> KNTVSIFALGPTITDDDEKMTLALLFLSHSLDNEKQHAQRAGFLVSLLSMAYANPELYLTTNGSNADVKYVIYMIEKDLKRQKYGGFVVKTREMIYEKTTEWIFGSDLDYDQETMLQNGRNNSTIEDLVHTFGYPSCLGALIIQIWIVLVKAITSISGLRKGFFTRLEAFRQDGTVQAGLVLSGDTVDQIGSIMRSQQSLVTLMVETLITMNTSRNDLTTIEKNIQIVGNYIRDAGLASFFNTIRYGIETRMAALTLSTLRPDINRLKALMELYLSKGPRAPFICILRDPIHGEFAPGNYPAIWSYAMGVAVVQNRAMQQYVTGRSYLDIDMFQLGQAVARDAEAQ;> MESDAKNYQIMDSWEEEPRDKSTNISSALNIIEFILSTD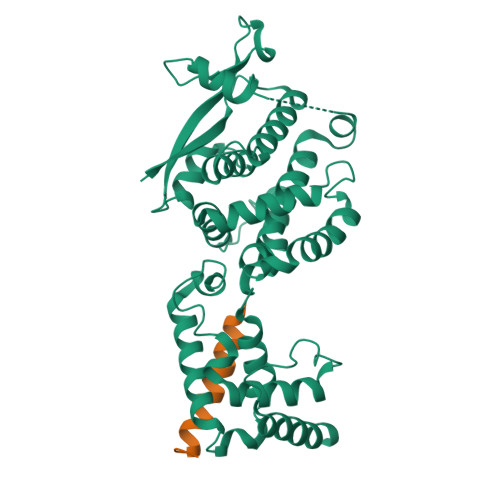PQE>MDHDFLKGQGDARSVRHIAIPAHRGLITDRNGEPLAVSTPVTTLWANPKELMTAKERWPQLAAALGQDTKLFADRIEQNAEREFIYLVRGLTPEQGEGVIALKVPGVYSIEEFRRFYPAGEVVAHAVGFTDVDDRGREGIELAFDEWLAGVPGKRQVLKDRRGRVIKDVQVTKNAKPGKTLALSIDLRLQYLAHRELRNALLENGAKAGSLVIMDVKTGEILAMTNQPTYNPNNRRNLQPAAMRNRAMIDVFEPGSTVKPFSMSAALASGRWKPSDIVDVYPGTLQIGRYTIRDVSRNSRQLDLTGILIKSSNVGISKIAFDIGAESIYSVMQQVGLGQDTGLGFPGERVGNLPNHRKWPKAETATLAYGYGLSVTAIQLAHAYAALANDGKSVPLSMTRVDRVPDGVQVISPEVASTVQGMLQQVVEAQGGVFRAQVPGYHAAGKSGTARKVSVGTKGYRENAYRSLFAGFAPATDPRIAMVVVIDEPSKAGYFGGLVSAPVFSKVMAGALRLMNVPPDNLPTAKLVPRG[2x]

Subclass B3 PBP (known as PBP3 in Escherichia coli and encoded by the ftsI gene) is active during cell division and localizes to a multiprotein complex termed the divisome, where it functions in PG synthesis in concert with the division-specific glycosyltransferase FtsW. PBP3 consists of three major domains: the N-terminal transmembrane helix anchors the protein in the cell membrane, while the C-terminal transpeptidase domain (TPd) is the catalytic module of PBP3 and mediates cross-linking of PG chains by ω-peptide linkages between d-Ala and meso-diaminopimelic acid (m-DAP) residues on opposing peptide chains. The catalytic serine acting as a nucleophile in the transpeptidation mechanism is also able to react with β-lactam antibiotics because of their structural similarity with the d-Ala-d-Ala motif; the resulting covalent intermediate, however, has a very long half-life (with turn-over constant k3 ~ 10−4 M−1s−1 or less), effectively leading to irreversible inactivation. AiCuris previously reported on the development of a novel monobactam (AIC499), which shows remarkable inhibitory activity against PBPs of Gram-negative bacteria, and good antibacterial activity, even against clinical isolates harboring several β-lactamase classes.

In addition to the apo structures, PaPBP3ΔTM was produced and crystallized in the presence of AIC499; crystals belonged to space group P 21 21 21 with two copies per asymmetric unit and yielded diffraction data extending to a resolution of 1.7 Å. For the complex with the E. coli protein, the AIC499 molecule is covalently associated with PaPBP3ΔTM via the catalytic serine (S294) side chain. In the active site environment, the β3-β4 loop as well as the β5-α11 loop appear quite flexible, despite the presence of the ligand, as evidenced by high B-factors and often discontinuous electron density. Nevertheless, we note that strands β3 and β4 clearly bend towards the active site, supporting some interactions of their side chains with the AIC499 molecule, most importantly R489 (see below). More importantly, helix α11 is N-terminally extended by more than one turn in both chains, which again allows additional contacts with the ligand. The terminal sulfate group (R2) is hydrogen bonded to the side chains of K484, S485, and T487 (the region of the third signature motif). The amino-thiazole (R4) is well stabilized, engaging in three hydrogen bonds with the side chain of E291 (specifically, one of its alternate conformations) and the backbone of R489. Unlike the situation in the EcPBP3ΔTM:AIC499 complex, the amino-thiazole does not form a parallel π-π stack with Y409 (equivalent to Y419 in EcPBP3) but a displaced T-stack. The carboxyl group of the linker (R5) forms hydrogen bonds to the guanidinium group of R489, and the phenyl ring of the head group (R1) is close to the aliphatic side chain of V333.>[2x]PIPSAEIFEDFLDWYTSGKAGEEIIESTDKRVEAIVEELGGELTEEMKEALAMARAAMAAFEKEGDVFRLASVGATAALMVWFHLRNIPLAGIARAWLLMLAQLEAGADVDTALAAAAEVLREYGVSEELVAAAAAEARALVESARRRGLTPFELASLAALAAARLLFTARNNPLAKIIQAALDLYNRTVDMSTEEAVEAALEAMKELGASEESLERL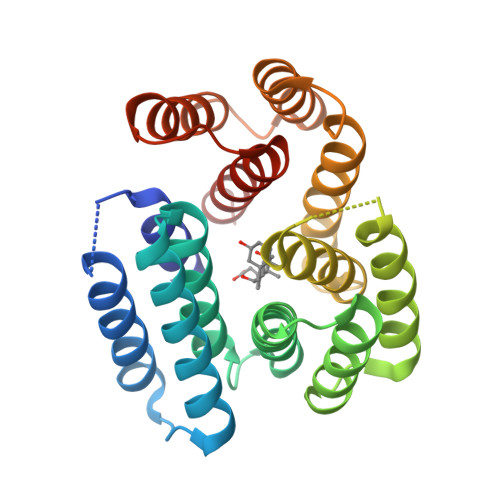KELVESARKRGIELTPFEVALLAYYVLVLDYLKKS> AAIHRTQLWFHGRISREESQRLIGQQGLVDGLFLVRESQRNPQGFVLSLCHLQKVKHYLILPSEEEGRLYFSMDDGQTRFTDLLQLVEFHQLNRGILPCLLRHCCT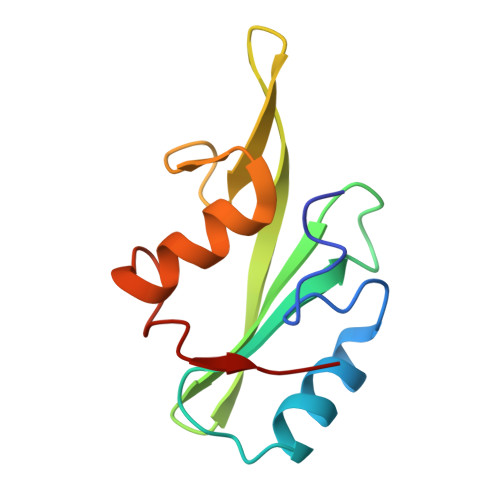R>ETGQTLAANIWSDKTTAQNEPINLTNANAPIKNAKNLNSTITNVAAFDTKLNHLLVDTITGRVFVGGVNRLYQLSPDLELSETVKTGPQNDSVECSILDCPLNAVRSPTDNYNKVLLIDRATSRLIACGSLFQGTCTVRNLQNVSIIEHEVPDAVVANDANSSTVAFIAPGPPQHPVTNVMYVGVTYTNNSPYRSEIPAVASRSLEKTKMFQIASSAVTTGTRTFINSYARETYFVNYVYGFSSERFSYFLTTQLKHSHHSSPKEYITKLVRICQEDSNYYSYTEIPVECISDAQGGTKFNLVQAGFLGKPSSDLAQSLGISIQDDVLFAVFSKGEGNTPTNNSALCIYSLKSIRRKFMQNIKSCFNGSGMRGLDFISPSMPCVLTKLQTIGEDFCGLDVNSPLGGETPITSVPVAMFNTKLTSVAATSTSGYTVVFVGTSDGFLKKVVIESSSIANEYASFAVDLGSEINRDMQFDNQNLYIYVMSKTKVSKVKVFDCSDYKTCGDCLGARDPYCGWCSLENKCSPRSNCQDDANDPLYWVSYKTGKCTTITSVVPHQLQRTTARTLELIIDHLPQLKENLICAFTTEDKALFTNATKKRNGVNCTTPRTDMLPQIEQGKHHFTAKLSVRTRNGPDLVSTDFTFFDCSTHSSCTRCVSSEFPCDWCVEAHRCTHDTAENCRNDILVTGVSRIGPSYRSGPGFCPTGTKHHHHHH[2x];>ETGDVKPDLQTKQDKVLAHFIGNSTDYFKILDHNDEFVLVGAKDVIYNVSLNGLKEIARLEWHSTDADRELCALKGKHEWDCHNYLRVYALRPNGEVLLCGTNSYKPRCRHYTPVEVSSEEAGSAGHAHAMRYEVSRDVEAQGLCPYSPAHNSTYAFADGHLYSATVADFSGGDPLIYRENLRTEQYDLKQLNQPDFVGAIERNGYVLFFFRELSMEVMNFGKAVYSRVARVCKNDRGGPYSHGKSWTSFLKARLNCSVPGEFPFYFDEIQAISPIVESGSKSLIYAVFTTSVNAIPGSAVCAFNVDDILAAFDGEFKSQKDSQSHWLPVEREQVPKPRPGQCVEDSRTLTSIAVNFIKNH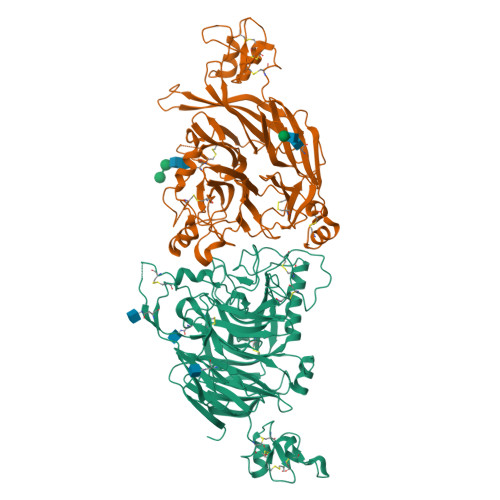PLMEEAVPAVHGRPLLTKVNLHHRLTAIAVHPQVKSLSGAYYDVIYSGTDDGKVTKFINILSTHPNSTVDRLKTVVISEMQVLPLGTPIRELVISTSKNSLVVVSDGSLVSVPLHHCSHIVDCLGCLSLQDPICAWDLQTHECKNLATSQHKFGTKTYLQSLNSTKKAAALLCPHIPRDAPGAETVSFVTMAPPPTEEQKLLYSNVGSGTKHHHHHH[2x]1-[PHENYL-(4-PHENYLPHENYL)-METHYL]IMIDAZOLE | C22 H18 N2 | 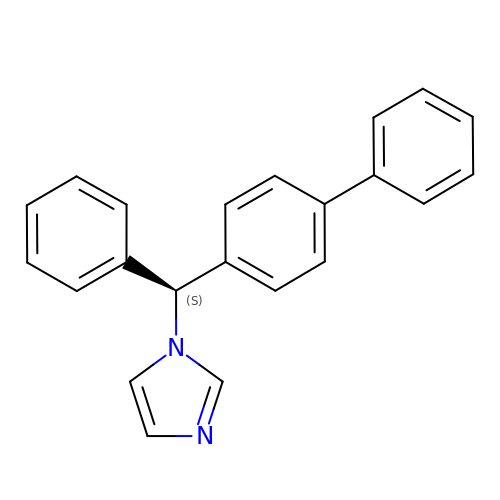OCAPBUJLXMYKEJ-QFIPXVFZSA-N2',5'-dideoxy-5'-[(diphenylmethyl)amino]uridine 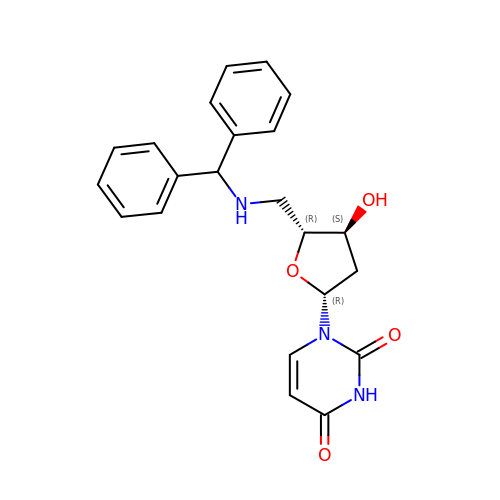| C22 H23 N3 O4 | JJVBLAPDVHVENR-NLWGTHIKSA-N> EA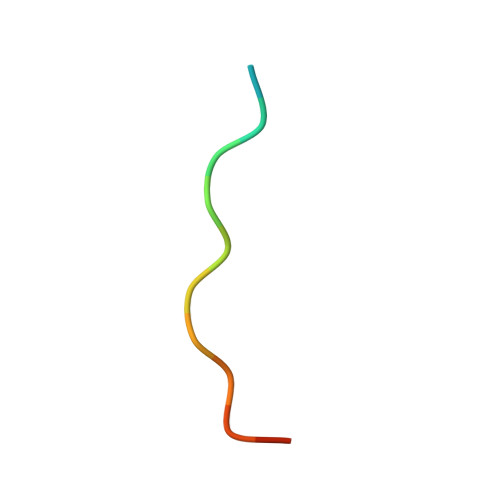MPPTLPHRDWKD> HHHHHHFNLPPGNYKKGDTHIQFQISPEGNGEVLLKSTETGQYLRINPDGTVDGTRDRSDT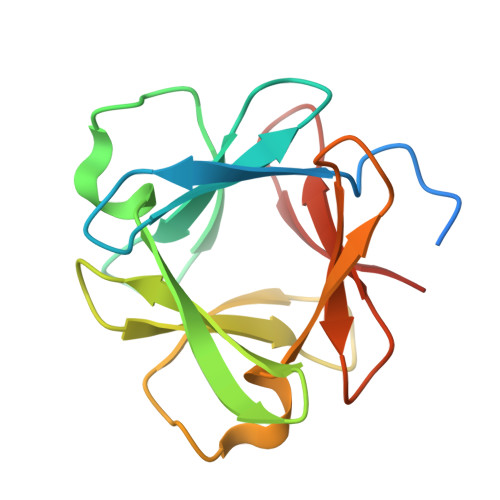HIQFQISPEGNGEVLLKSTETGQYLRINPDGTVDGTRDRSDTHIQFQISPEGNGEVLLKSTETGQYLRINPDGTVDGTRDR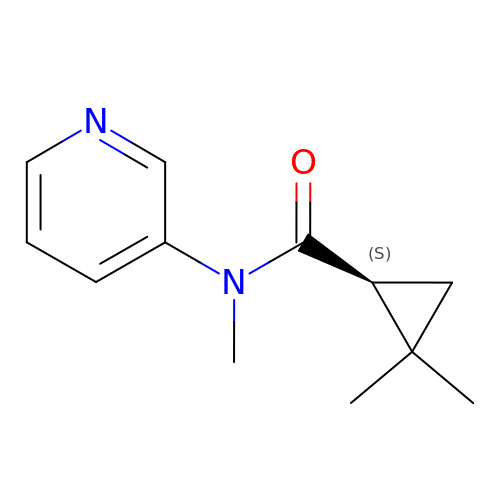(1S)-N,2,2-trimethyl-N-(pyridin-3-yl)cyclopropane-1-carboxamide | C12 H16 N2 O | TVMZQESCEGRMKC-SNVBAGLBSA-N> ASSVNELENWSKWMQPIPDSIPLARISIPGTLDSGTFKLQNPIKQVWGMTQEYDFRYQMDHGARIFDIRGRLTDDNTIVLHHGPLYLYVTLHEFINEAKQFLKDNPSETIIMSLKKEYEDMKGAEDSFSSTFEKKYFVDPIFLKTEGNIKLGDARGKIVLLKRYSGSNEPGGYNNFYWPDNETFTTTVNQNANVTVQDKYKVSYDEKVKSIKDTMDETMNNSEDLNHLYINFTSLSSGGTAWNSPYYYASYINPEIANYIKQKNP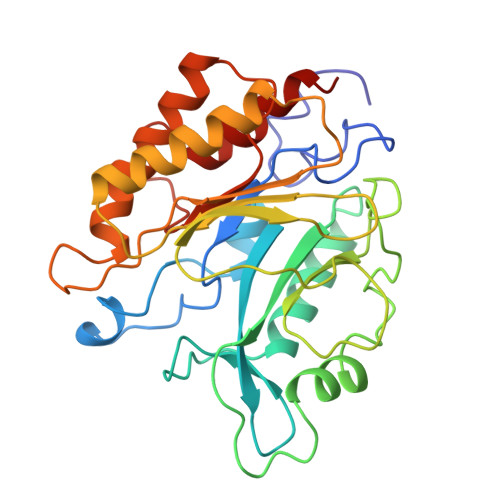ARVGWVIQDYINEKWSPLLYQEVIRANKSLIKE>GAMGSMATRIAILGAGPSGMAQLRAFQSAQEKGAEIPELVCFEKQADWGGQWNYTWRTGLDENGEPVHSSMYRYLWSNGPKECLEFADYTFDEHFGKPIASYPPREVLWDYIKGRVEKAGVRKYIRFNTAVRHVEFNEDSQTFTVTVQDHTTDTIYSAAFDYVVCCTGHFSTPYVPEFEGFEKFGGRILHAHDFRDALEFKDKTVLLVGSSYSAEDIGSQCYKYGAKKLISCYRTAPMGYKWPENWDERPNLVRVDTENAYFADGSSEKVDAIILCTGYIHHFPFLNDDLRLV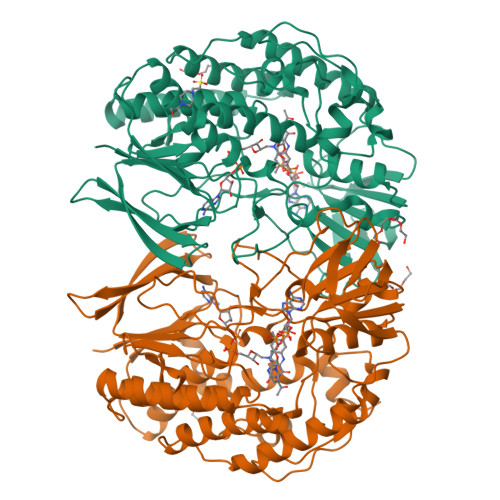TNNRLWPLNLYKGVVWEDNPKFFYIGMQDQWYSFNMFDAQAWYARDVIMGRLPLPSKEEMKADSMAWREKELTLVTAEEMYTYQGDYIQNLIDMTDYPSFDIPATNKTFLEWKHHKKENIMTFRDHSYRSLMTGTMAPKHHTPWIDALDDSLEAYLSDKSEIPVAKEA[4x]> MEIKKGLEDVYVKETEITYIDGELGRLYYRGYSIYDLAEFSNFEEVSYLILYGKLPNREELNWFQEKLREERYLPDFIIKFLREVRKDAQPMDILRTAVSLLGIEDSKNDERTDIKGIKLISKFPTIVANYARLRKGLDIIEPDPKLSHSENFLYMLYGDRPNEIKSKAMDVTLILHIDHEMNASTFASLVVASTFSDLYSSIVAGISALKGPLHGGANYEALKMFKEIGSPEKVNDYILNRLSNKQRIMGFGHRVYKTYDPRARILKQYAKLLAEKEGGEIYTLYQIAEKVEEIGIKYLGPKGIYPNVDFFSSIVFYSLGFEPDFFPAVFASARVVGWVAHIMEYIKDNKIIRPKAYYKGEIGKKYIPIDSR

Citrate synthase (CS, EC 2.3.3.1), an enzyme involved in the TCA cycle, catalyzes the condensation of oxaloacetate and acetyl-coenzyme-A (CoA) to form citrate and CoA. Thermoacidophilic archaeon Sulfolobus tokodaii strain 7, which grows optimally at 75°C and pH 3, has two genes encoding two distinct isozymes of hypothetic CS. One of them encoded by an open reading frame (ORF) ST1805 is termed ST1805-CS, and the other, encoded by the ORF ST0587, is termed ST0587-CS. We confirmed these two isozymes to function in high temperatures as CS and determined the crystal structures of them at resolutions of 2.0 Å and 2.7 Å, respectively.

On the other hand, ST0587-CS exhibits 51% sequence identity with CS from hyperthermophilic archaeon Pyrococcus furiosus (PF-CS). ST0587-CS crystallized into an orthorhombic crystal belonging to P41212 that diffracted X-rays up to 2.7 Å resolution. In this crystal form, the asymmetric unit contains one monomer. This citrate synthase also forms a dimeric structure, the 2-fold axis of which coincides with the crystallographic 2-fold axis. The final model is comprised of 373 amino acid residues and 40 water molecules. As observed for ST1807-CS, each subunit is subdivided into a large domain with 11 α-helices (C-G, I-M, and S helices, residues 1–212 and 321–373) and a small domain with five α-helices (N-R helices, residues 213–320). The N-terminal region is folded into three strands (residues 18–21, 26–29, and 32-33), forming an antiparallel β-sheet, whereas an intersubunit β-sheet found in ST1805-CS is absent in ST0587-CS. In the structure of ST0587-CS, six putative substrate-binding residues (His180, His215, His254, Arg263, Arg335, and Arg354′) were also structurally conserved. The numbers of ion pairs composed of residues of opposite charge situated within 4.0 Å were 36 and 55 in each dimer of ST1805-CS and ST0587-CS, respectively. In ST0587-CS, an ion pair network was organized by four residues, Asp93 and Arg96 in G helix, Lys211 in MN loop, and Asp198′ in L′M′ loop of neighboring subunit, and continued into hydrophobic center of the helix bundle.> MELKNSISDYTEAEFVQLLKEIEKENVAATDDVLDVLLEHFVKITEHPDGTDLIYYPSDNRDDSPEGIVKEIK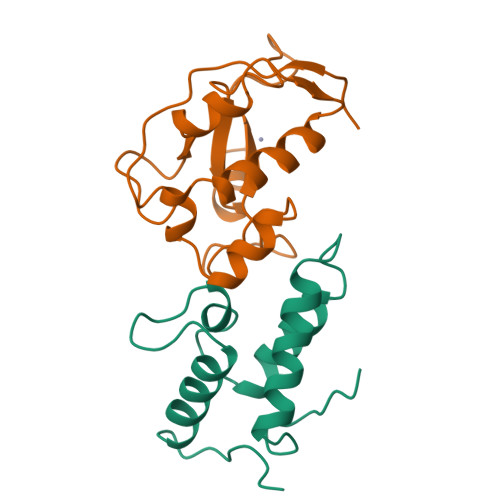EWRAANGKPGFKQG;> ERFAREPMAAGHRMWQMAGLKAQRAQTDVNNKKAAFDAAAKEKSDADVALSSALERRKQKENKEKDAKAKLDKESKRNKPGKATGKGKPVNNKWLNNAGKDLGSPVPDRIANKLRDKEFKSFDDFRKKFWEEVSKDPELSKQFSRNNNDRMKVGKAPKTRTQDVSGKRTSFELHHEKPISQNGGVYDMDNISVVTPKRHIDIHRGK>[60x]MLAQVLRRQALQHVRLARAAAPSLTR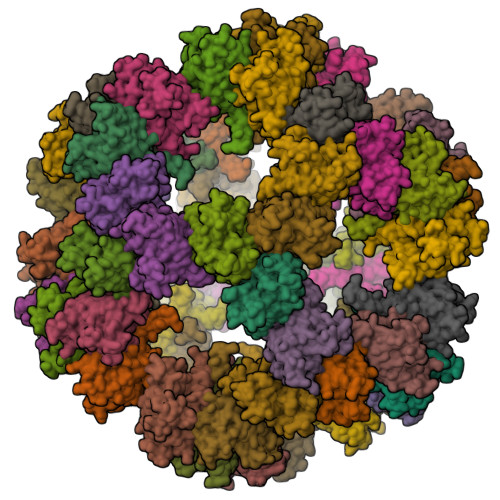WYASYPPHTIVKMPALSPTMTSGNIGAWQKKPGDAITPGEVLVEIETDKAQMDFEFQEEGVLAKILKETGEKDVAVGSPIAVLVEEGTDINAFQNFTLEDAGGDAAAPAAPAKEELAKAETAPTPASTSAPEPEETTSTGKLEPALDREPNVSFAAKKLAHELDVPLKALKGTGPGGKITEEDVKKAASAPAAAAAAPGAAYQDIPISNMRKTIATRLKESVSENPHFFVTSELSVSKLLKLRQALNSSAEGRYKLSVNDFLIKAIAVACKRVPAVNSSWRDGVIRQFDTVDVSVAVATPTGLITPIVKGVEAKGLETISATVKELAKKARDGKLKPEDYQGGTISISNMGMNPAVERFTAIINPPQAAILAVGTTKKVAVPVENEDGTTGVEWDDQIVVTASFDHKVVDGAVGAEWMRELKKVVENPLELLL> GAGCAGACCTGACGGCACTCA;> CCGTCA;> TCTGAGTG;> GGTCTGC

In this work, we exhaustively probe the ability of all 36 immobile HJ sequences to form DNA crystals in two different designed systems. Three separate self-assembling DNA crystal systems are described in this report: the “4 × 5” and “4 × 6” designs (collectively referred to as the 4 × N systems), and a third construct with a “scrambled” sequence variant of the 4 × 6 lattices. Self-assembly was mediated by three constituent oligonucleotides: (S1) containing four sequence repeats of either 5 or 6 bases; (S2) composed of 21 bases containing complementary regions to both (S1); and (S3) which forms the second junction crossover. The HJ serves as the fundamental component at the core of each unit, and the ultimate assembly of the full lattice is facilitated by the complementary 2-base sticky ends that tail each duplex.

Seventeen of the 36 junctions successfully crystallized, a 47% success rate. Unlike the 4 × 5 motif, nearly all of the 4 × 6 junction sequences had a strong preference for crystallization in buffers containing ≥2.0 M salts (e.g., LiCl, Li2SO4, KCl, and NaCl), with the majority preferring slightly basic pH conditions in cacodylic acid. The average cell constants for the P32 crystals were a = b = 68.29 Å c = 55.68 Å. Pos1 and 2 were readily observable in the electron density maps at either one or both of these conserved sites in a significant number of the structures, with no apparent respect to motif or symmetry. Only cobalt could account for the different peaks in the Fo–Fc maps in J25, whereas in J34, and J22 and J23 in the 4 × 6 and 4 × 6 scramble systems, respectively, contained Mg2+. The modeled ions were readily superimposable, and well-coordinated at Pos1 & 2.>SMLNVGATAPDFTLRDQNQQLVTLRGYRGAKNVLLVFHPLAFTGICQGELDQLRDHLPEFENDDSAALAISVGPPPTHKIW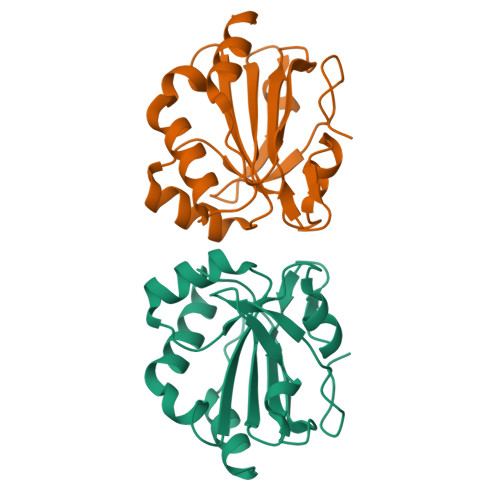ATQSGFTFPLLSDFWPHGAVSQAYGVFNEQAGIANRGTFVVDRSGIIRFAEMKQPGEVRDQRLWTDALAALT[2x]> MNYNNKILVSESGLSQKHLIHGDEELFQHELKTIFARNWLFLTHDSLIPAPGDYVTAKM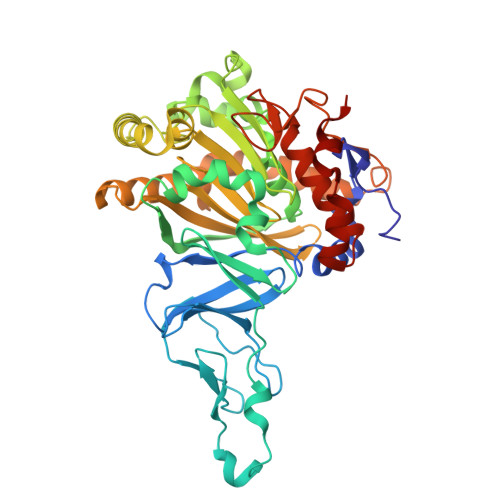GIDEVIVSRQNDGSIRAFLNVCRHRGKTLVSVEAGNAKGFVCSYHGWGFGSNGELQSVPFEKDLYGESLNKKCLGLKEVARVESFHGFIYGCFDQEAPPLMDYLGDAAWYLEPMFKHSGGLELVGPPGKVVIKANWKAPAENFVGDAYHVGWTHASSLRSGESIFSSLAGNAALPPEGAGLQMTSKYGSGMGVLWDGYSGVHSADLVPELMAFGGAKQERLNKEIGDVRARIYRSHLNCTVFPNNSMLTCSGVFKVWNPIDANTTEVWTYAIVEKDMPEDLKRRLADSVQRTFGPAGFWESDDNDNMETASQNGKKYQSRDSDLLSNLGFGEDVYGDAVYPGVVGKSAIGETSYRGFYRAYQAHVSSSNWAEFEHASSTWHTELTKTTDR Homologous to both U2AF65 and the yeast Mud2p, the Poly(U)-binding splicing factor 60 kDa (PUF60) shares domain features with U2AF65 by also containing two central RRMs and a C-terminal UHM. The most noticeable differences of domain structure between PUF60 and U2AF65 include the lack of the RS domain in PUF60 and a highly extended linker connecting the second RRM and UHM in PUF60. Although both U2AF65 and PUF60 are general splicing factors, the PUF60/U2AF65 ratio in cells influences alternative splicing patterns, suggesting PUF60 is implicated in alternative splicing. PUF60 appears to promote splicing at a weak 3’ splice site.

(A) The structure of PUF60 RRMs in the absence of oligonucleotide was determined to 2.8 Å. A dimer is observed in the crystal structure, although the protein is monomeric in solution when unbound. (B) The dimer interface observed in the crystal structure of unbound PUF60 RRMs is fairly similar to that seen in the dAdML3’-bound structure, with Lys-201 from each subunit crossing each other to span the dimer interface, suggesting that the dAdML3’ takes advantage of an inherent capability of the protein to dimerize, so that the higher oligomeric state is induced in solution in the presence of the oligonucleotide. ssDimerization of unbound PUF60 RRMs is not observed in solution, and therefore must be due to high concentration of protein in the crystal. The similarity of the dimeric interface of the unbound protein to that found when the protein is bound to dAdML3’ indicates that the propensity for dimerization is inherent in the protein before it encounters nucleic acid, and the nucleic acid enhances this propensity to dimerize such that dimerization can occur at lower protein concentration in the presence of nucleic acid. None of the residues in the dimeric interface are close enough for hydrogen bonding, except for the amide nitrogen of each Val-202 donating a hydrogen bond to the carbonyl oxygen of Val-202 of the opposite subunit. However, in the unbound PUF60 RRMs structure, most of the residues in the dimeric interface are not close enough to hydrogen bond. Although the dimerization is unrealized at normal protein concentration, the interaction of uracil in the oligonucleotide with Lys-201 adds one more hydrogen bond, which would make dimer formation more energetically favorable. However, in the absence of nucleotide, PUF60 RRMs does not dimerize, and neither does PUF60 RRMs+UHM.

>GSHMASMTGGQQMGRGSAAQRQGALAIMSRVYVGSIYYELGEDTIRQAFAPFGPIKSIDMSWDSVTMKHKGFAFVEYEVPEAAQLALEQMNSVMLGGRNIKVGRPSNIGQAQPIIDQLAEEARAFNRIYVASVHQDLSDDDIKSVFEAFGKIKSATLARDPTTGKHKGYGFIEYEKAQSSQDAVSSMNLFDLGGQYLRVGKAVTPPMPLLTPATPG[2x]>[2x]MASPAVRKAISDAALQYAKPEGKIFQYGTAGFRMKADLLNTVVYAVGLLATLRSKKLSGQWIGVMVTASHNPAEDNGVKLVDPMGEMLEAEWEAYAT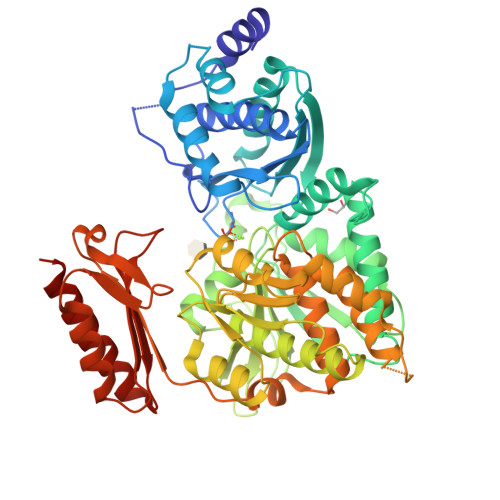KLANAPLENIGDVYDELVKEIDVSMENPARVVFARDTRASGSRLIGVLSAALTATEAEFIDMKFMTTPQLHYVVRCKNTLGTQYEYGEPTEQGYYEKLAAAFKRVMRGVKVKGSLTVDCANGVGGPKLRELIKYLPEDTGLDIKIVNDDVINPDSLNFECGADYVKTKQRAPPSSKASILDRCASLDGDADRILYYFLDEGNVFRLLDGDRIATLAASFIGDLARSAGIAQKLKIGVVQTAYANGSSTEYIEKVLKLPSVCTNTGVKHLHHAAMRFDVGVYFEANGHGTITFSENALKTIKNTEPQSPAQQRSLECLQALTDLINQAVGDAISDMLLVEAILAHKGWTPKEWLATYTDLPSRLVRVEVAERSIFKAYDAERKLESPPGLQAKIDSLQSRYNKGRSFARASGTEDAVRVYAEAASRSEADDLATRVANAVRDAGTVKEILQAS>[2x]MNKPSFLLVGLLVVSGVLGAAETKVKYPDGFRSWYHVKSMVIQPGHPLENPF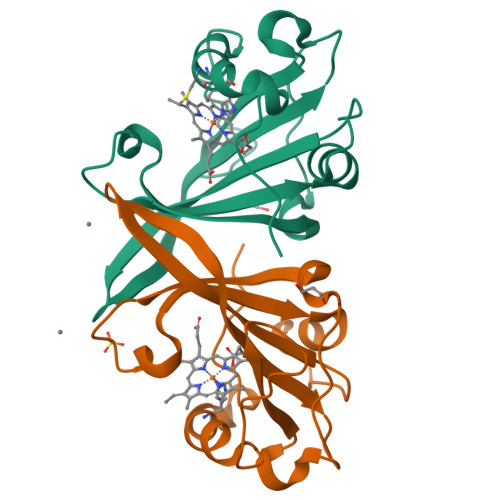GGIHHVYANAEAIQGLRGGNYPDGAVLVFDLFDYQEDNHALVEGKRKLIGVMERDAKRFSATGGWGYEGFGEGKPDKRLVTDGGQGCFGCHAAQKESQYVFSRLRD> GNNS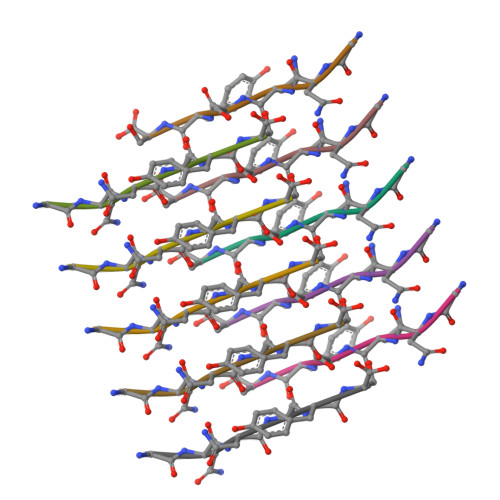YS>MGLQARSHSQARLDNLLNQELPAQVKGLAAHINLSLSQDLAISESLANSYFIEQWVREGLPEERQNDIAAYLARLMEQLDTELLFIAAQHQGRGYYFQLRNGEFLQRIIQPPGSEDDWYYHFTDSDNAYELNLDSDTFSPD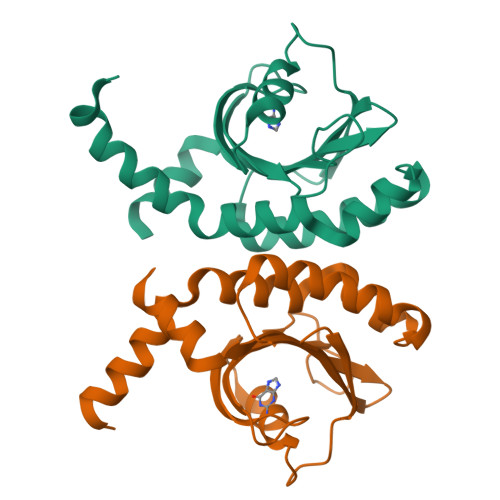DAFVYVNYRSTVNAANGRPLVVAGAGLDLSQMASLIDDFRLGGSGHASLLSAEGELLVRSGEAKRSDESAPTVATATEALPEQASQRLLQNEQLQVHEATRDGQEVLVSTIWLPELQRYLMVEVDKKAYLASTHERFLELEHHHHHH[6x]> GSHMAKTYDYLFKLLLIGDSGVGKTCVLFRFSEDAFNSTFISTIGIDFKIRTIELDGKRIKLQIWDTAGLERFRTITTAYYRGAMGIMLVYDITNEKSFDNIRNWIRNIEEHASADVEKMILGNKC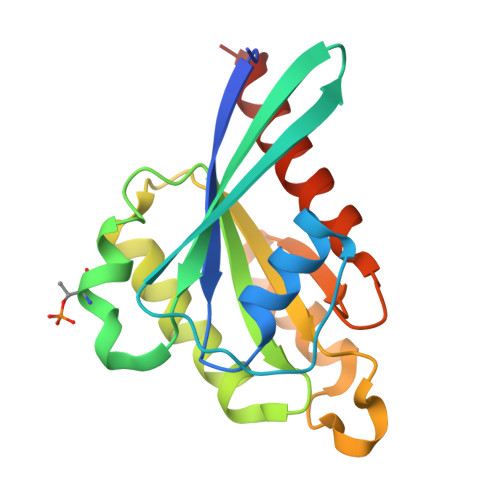DVNDKRQVSKERGEKLALDYGIKFMETSAKANINVENAFFTLARDIKAKMDKKLEGNS>[2x]GSEAIAKYDFKATADDELSFKRGDILKVLNEESDQNW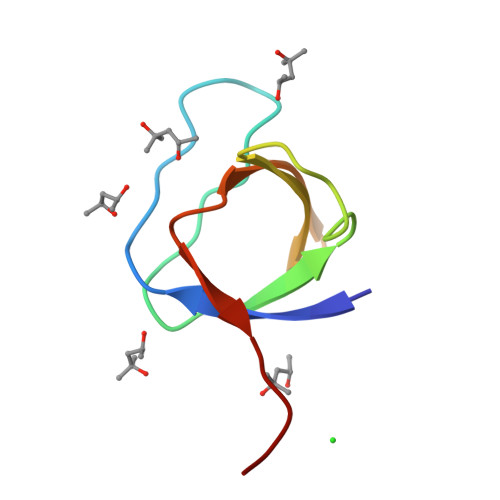YKAELNGKDGFIPKNYIEMKPHPG>[2x]MLANENSLLTMFRELGSGKLPLQIEQFERGKTIFFPGDPAERVYLLVKGAVKLSRVYESGEEITVALLRENSVFGVLSLLTGQRSDRFYHAVAFTPVQLFSVPIEFM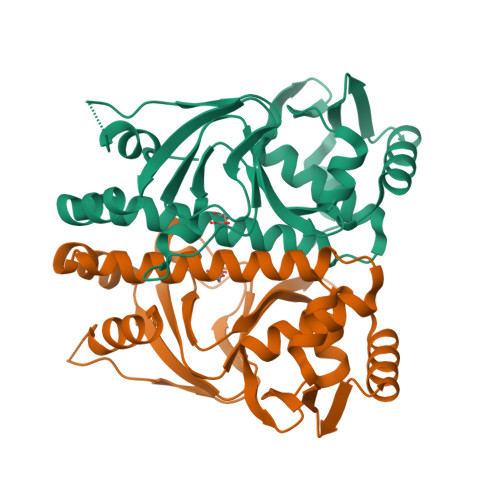QKALIERPELANVMLQGLSSRILQTEMMIETLAHRDMGSRLVSFLLILCRDFGIPSPDGITIDLKLSHQAIAEAIGSTRVTVTRLLGDLRESKLIAIHKKRITVFNPVALSQQFS2,3,4,6-tetrahydroxy-5H-benzo[7]annulen-5-one | C11 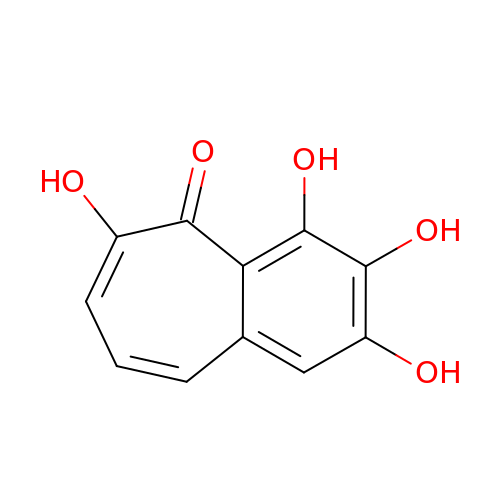H8 O5 | WDGFFVCWBZVLCE-UHFFFAOYSA-N>SHMSLTPDQIVAALQERGWQAEIVTEFSLLNEMVDVDPQGILKCVDGRGSDNTQFCGPKMPGGIYAIAHNRGVTTLEGLKQITKEVASKGHVPSVHGDHSSDMLGCGFFKLWVTGRFDDMGYPRPQFDADQGAK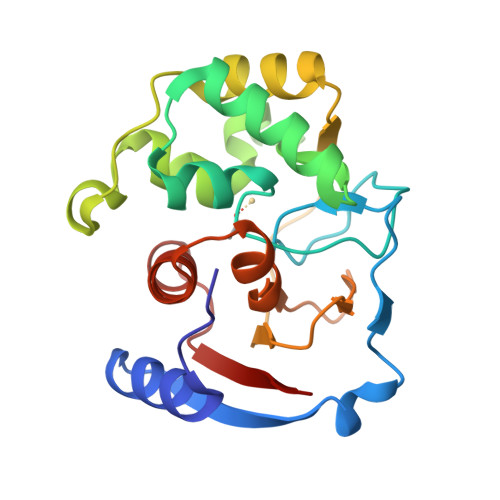AVENAGGVIEMHHGSHAEKVVYINLVENKTLEPDEDDQRFIVDGWAAGKFGLDVPKFLIAAAATVEMLGGPKKAKIVIP[2x]> SKGENSKLNPWAVVGFIDAEGSFMVRVRKNSKYKTGWLVVAIFSVTVDKKDLFLLESLKTFFGGLGSIKKSGNSTFSYRIESSEQLTKIILPFFDKYSLITEKLGDYLLFKKVLELMGTKEHLTQRGLEKIVSLKASINKGLSEELQAAFPQCVPTPRPEINNKNIPDPFWLAGFVSGDGSFKSILKKSESIKVGF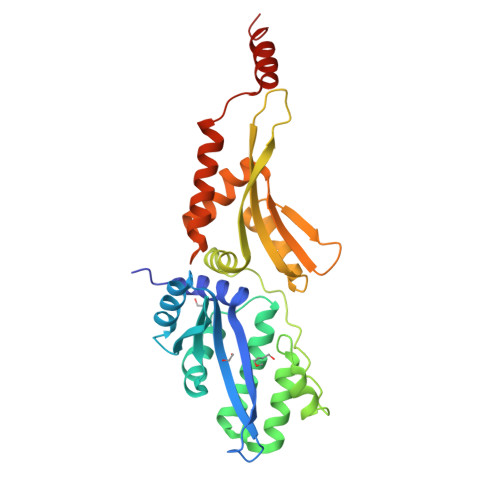QSILVFQITQHARDVKLMESLISYLGCGFIEKDSRGPWLYYTVTNFSDIQGKIIPFFHQYKIIGSKYGDYQDWCKIALIMQNKNHLTPEGLNEIRALKGGMNKGRL>[3x]MKTIKDRIAKWSAIGLLSAVAATAFYAPSASAHGEKSQAAFMRMRTIHWYDLSWSKEKVKINETVEIKGKFHVFEGWPETVDEPDVAFLNVGMPGPVFIRKESYIGGQLVPRSVRLEIGKTYDFRVVLKARRPGDWHVHTMMNVQGGGPIIGPGKWITVEGSMSEFRNPVTTLTGQTVDLENYNEGNTYFWHAFWFAIGVAWIGYWSRRPIFIP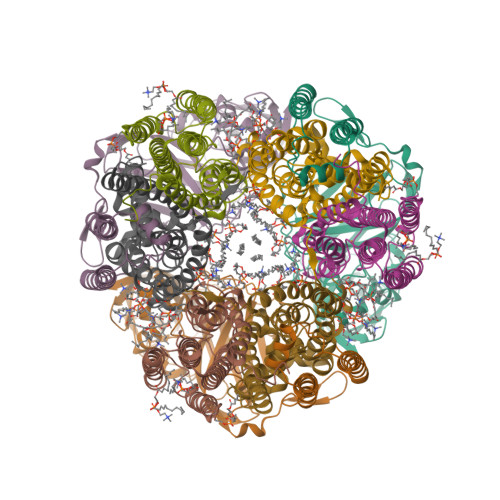RLLMVDAGRADELVSATDRKVAMGFLAATILIVVMAMSSANSKYPITIPLQAGTMRGMKPLELPAPTVSVKVEDATYRVPGRAMRMKLTITNHGNSPIRLGEFYTASVRFLDSDVYKDTTGYPEDLLAEDGLSVSDNSPLAPGETRTVDVTASDAAWEVYRLSDIIYDPDSRFAGLLFFFDATGNRQVVQIDAPLIPSFM;>MSAAQSAVRSHAEAVQVSRTIDWMALFVVFFVIVGSYHIHAMLTMGDWDFWSDWKDRRLWVTVTPIVLVTFPAAVQSYLWERYRLPWGATVCVLGLLLGEWINRYFNFWGWTYFPINFVFPASLVPGAIILDTVLMLSGSYLFTAIVGAMGWGLIFYPGNWPIIAPLHVPVEYNGMLMSIADIQGYNYVRTGTPEYIRMVEKGTLRTFGKDVAPVSAFFSAFMSILIYFMWHFIGRWFSNERFLQST[3x];>[3x]MAATTIGGAAAAEAPLLDKKWLTFALAIYTVFYLWVRWYEGVYGWSAGLDSFAPEFETYWMNFLYTEIVLEIVTASILWGYLWKTRDRNLAALTPREELRRNFTHLVWLVAYAWAIYWGASYFTEQDGTWHQTIVRDTDFTPSHIIEFYLSYPIYIITGFAAFIYAKTRLPFFAKGISLPYLVLVVGPFMILPNVGLNEWGHTFWFMEELFVAPLHYGFVIFGWLALAVMGTLTQTFYSFAQGGLGQSLCEAVDEGLIAK However, a dormant state in Firmicutes can be recapitulated in the laboratory. This paper describes the first structure of a group of peptidoglycan cleaving enzymes from Firmicutes, called stationary phase survival proteins (Sps), that are involved in survival in the stationary phase and are analogous to the resuscitation promoting factors (Rpfs) from Actinobacteria. In this paper we present three high-resolution crystal structures of YuiC, an Sps protein from B. subtilis. The overall fold of each domain of the symmetric dimer consists of a mixed direction six stranded double psi beta barrel surround by five helices. In all the structures, the final two helices and the last strand of the beta barrel of each half are supplied by the other chain in the dimer.

Crystallisation of YuiC in the presence of NAG gives a structure with a single well defined NAG per chain. The NAG in + NAG superimposes with the −2 position in the chitohexose in MltA. The interaction of the conserved D297 (MltA)/D151 (YuiC) with the N of the N-acetyl group of the NAG at the −2 position is conserved. Further hydrogen bonds to this sugar in YuiC are from the non-conserved K102 NZ to the N-acetyl carbonyl and O3 of NAG. The O3 hydroxyl in the −2 position forms a hydrogen bond to the backbone carboxyl of L111, which would prevent there being a N-acetylmuramicacid (NAM) at this position. The two ligand bound structures have good electron density for all residues, and superimpose very well with a RMSD 0.40 Å over 289 CA atoms of the dimer or 0.23 Å over 145 CA atoms of the pseudo monomer (formed by chain A 72–176 and chain B 177–216). MltA superimposes on the YuiC (+NAG) structure with an RMSD of 2.07 Å over 102 of the 146 modelled residues (72–217) in the pseudo monomer. Taking just the residues 166–178 from the two chains of + NAG using PISA 316 Å2 is buried between the two helices and surrounding linkers with no additional hydrogen bonds or salt bridges definitely formed in the dimer compared to two separate monomers. Intriguingly there is only room for one sugar site on the vacant + side of the cleavage in the + NAG and anhydro structure. The +2 sugar in the MltA superposition clashes with the third (domain swap) helix backbone. This would prevent the sugar chain being longer than +1 and so the dimer could only remove a terminal NAG (ie be an exo glycosidase).

>RLKALQQKQTQTTSAAEDKTKPLEEAFDWDEYPVQRVTATGYTAGAESTGKNPGDPLYGLTYSGVKVKRDLYSTVAADPSVFPIGTILFIPNYGLGVVADTGSAIKGNRLDLYFETVKDVYNEWGKKTLDVYVIKKGTGKITEDELEKLNETKSLQVFRNQYKTVKE[2x]>[2x]GHMTPANIAGMVVFIDPGHNGANDASIGR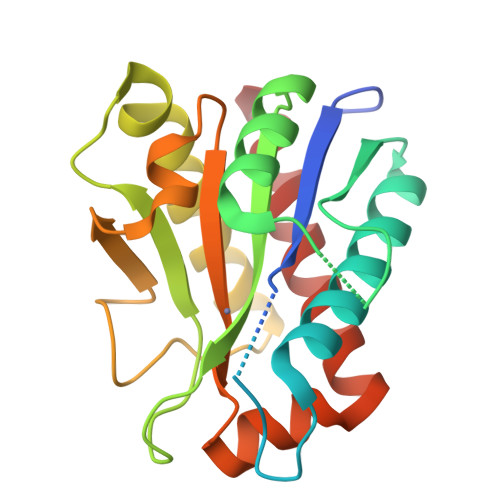QVPTGRGGTKNCQASGTSTNSGYPEHTFTWETGLRLRAALNALGVRTALSRGNDNALGPCVDERANMANALRPNAIVSLHADGGPASGRGFHVNYSAPPLNAIQAGPSVQFARIMRDQLQASGIPKANYIGQDGLYGRSDLAGLNLAQYPSILVELGNMKNPADSALMESAEGRQKYANALVRGVAGFLATQGQAR> APLVHHHHHHALDENLYFQGALADVSRPPHARKTGGSSPETKYDQPPKCDISGKEAISALSRAKSKHCRQEIGETYCRHKLGLLMPEKVTRFCPLEGKANKNVQWDEDSVEYMPANPVRIAFVLVVHGRASRQLQRMFKAIYHKDHFYYIHVDKRSNYLHRQVLQVSRQYSNVRVTPWRMATIWGGASLLSTYLQSMRDLLEMTDWPWDFFINLSAADYPIRTNDQLVAFLSRYRDMNFLKSHGRDNARFIRKQGLDRLFLECDAHMWRLGDRRIPEGIAVDGGSDWFLLNRRFVEYVTFSTDDLVTKMKQFYSYTLLPAESFFHTVLENSPHCDTMVDNNLRITNWNRKLGCKCQYKHIVDWCGCSPNDFKPQDFHRFQQTARPTFFARKFEAVVNQEIIGQLDYYLYGNYPAGTPGLRSYWENVYDEPDGIHSLSDVTLTLYHSFARLGLRRAETSLHTDGENSCRYYPMGHPASVHLYFLADRFQGFLIKHHATNLAVSKLETLETWVMPKKVFKIASPPSDFGRLQFSEVGTDWDAKERLFRNFGGLLGPMDEPVGMQKWGKGPNVTVTVIWVDPVNVIAATYDILIESTAEFTHYKPPLNLPLRPGVWTVKILHHWVPVAETKFLVAPLTFSNRQPIKPEEALKLHNGPLRNAYMEQSFQSLNPVLSLPINPAQVEQARRNAASTGTALEGWLDSLVGGMWTAMDICATGPTACPVMQTCSQTAWSSFSPDPKSELGAVKPDGRLR;> QEEEGAGGGQGG

The first enzyme in the pathway, peptide O-xylosyltransferase (XT, EC 2.4.2.26), catalyzes the transfer of xylose from uridine diphosphate (UDP)-α-D-xylose onto serine and thus determines the site(s) of GAG attachment on the core protein. XT1 and XT2 are type II transmembrane proteins consisting of a short amino-terminal region facing the cytosol, a single transmembrane helix, a stem region required for Golgi localization (Schön et al., 2006), a catalytic GT-A domain (Lairson et al., 2008, Müller et al., 2006), and a unique C-terminal domain of unknown function, termed “Xylo_C” in the Pfam database (Finn et al., 2008). XT1 has a two-lobed structure, with one lobe comprising the catalytic GT-A domain and the other comprising the Xylo_C domain. To better understand the initial step of GAG biosynthesis, we have determined crystal structures of human XT1 complexed with UDP-xylose and various PG-derived acceptor peptides.

We also prepared a ternary complex of XT1 with the sugar donor, UDP-xylose, and an inactive bikunin-derived peptide in which the acceptor serine was replaced by alanine. The complex of XT1 with UDP-xylose was obtained with the inactive peptide 2, in which the acceptor serine is mutated to alanine. Electron density for the xylose group was visible and refinement yielded a 4C1 chair conformation for the xylose group. However, residual difference density around the xylose and β-phosphate group, and the high B factors of the xylose atoms, suggest a mixed population of conformations or partial hydrolysis of UDP-xylose. The xylose group forms polar contacts with D494 and E529, and apolar contacts with W392 and W495. Of particular note is the close contact between the xylose C5 atom and the side chain of W392, which likely prevents binding of larger hexose and hexosamine sugars. In the ternary complex, continuous electron density was observed for 9 of the 12 amino acid residues of peptide 2. The peptide is bound within a cleft delimited on one side by the disulfide-bonded hairpin formed by residues 555–575, and on the other side by a loop containing a short α helix, the last turn of which constricts the width of the cleft (XT1 residues K461 and Q462). It is noteworthy that all but one of the 11 hydrogen bonds between peptide 2 and the GT-A domain involve the peptide's main-chain carbonyl and amide groups, i.e., they are not sequence specific. The structure of the Michaelis-like ternary complex with UDP-xylose and peptide 2 suggests that XT1 follows a direct-displacement SN2-like mechanism, similarly to other inverting GTs with a GT-A fold (Lairson et al., 2008).> SNAEKAVLIGEKEADITFVTWGSQKGPILDVIEDLKEEGISANLLYLKMFSPFPTEFVKNVLSS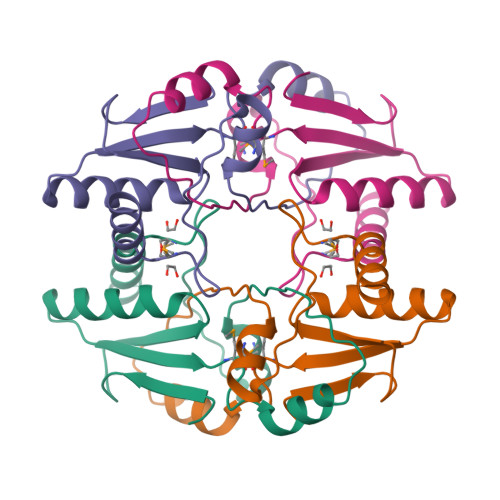ANLVIDVESNYTAQAAQMIKLYTGIDIKNKILKYNGRHMTEDEILKSAKEILNK2-(1H-pyrazol-3-yl)-1H-benzimidazole | C10 H8 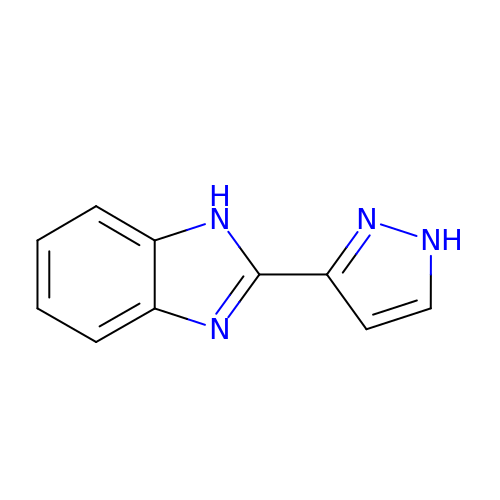N4 | IYTGPPNUOLLGBE-UHFFFAOYSA-N~{N}-[2-[[3-[3-[(4-azanylcyclohexyl)sulfamoyl]-4-methoxy-phenyl]-6-chloranyl-2-methyl-imidazo[1,2-b]pyridazin-8-yl]amino]ethyl]ethanamide | C24 H32 Cl N7 O4 S 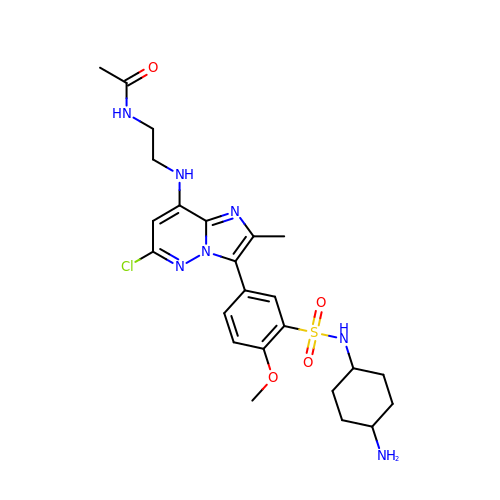| HORACVGDHNAIMC-IYARVYRRSA-N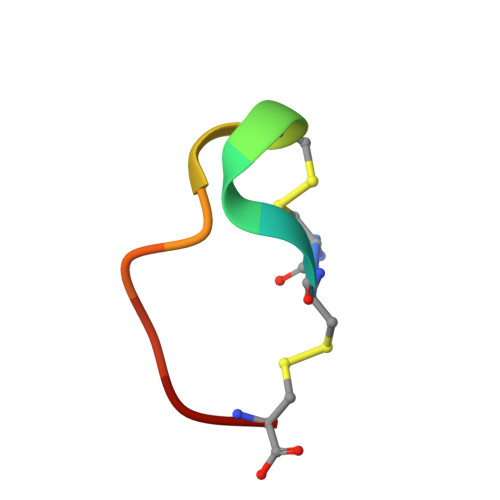> CCHPQCGAAYSC> MSSVDVLLTVGKLDASLALLTTQDHHVIEFPTVLLPENVKAGSIIKMQVSQNLEEEKKQRNHFKSIQAKILEKYGTH;> MNLFWPSETKKQNEIPGGDYTPGNSPSVQKGYQFLNRDIFKSCPRIMERQFGECLHNRTHLIKDLISSGNVGLGPIEIVHMSYLNKHEKEEFGEYFYVTGIEVSGPAMPVEFLEVLKSSKRISKNISNNIILTYCCFNFFSNLDIRIRYDADDTFQTTAIDCNKETTDLTMTEKMWEETFASSVIRAIITNTNPELKPPGL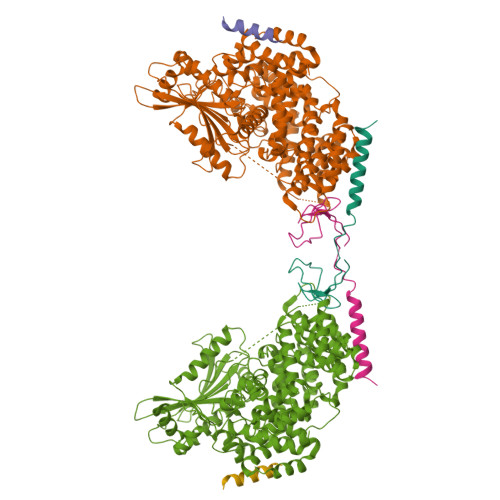VECPFYVGKDTISSCKKIIELLCRFLPRSLNCGWDSTKSMQATIVNNYLMYSLKSFIAITPSLVDFTIDYLKGLTKKDPIHDIYYKTAMITILDHIETKELDMITILNETLDPLLSLLNDLPPRDADSARLMNCMSDLLNIQTNFLLNRGDYELALGVSNTSTELALDSFESWYNLARCHIKKEEYEKALFAINSMPRLRKNDGHLETMYSRFLTSNYYKKPLNGTREHYDLTAMEFTNLSGTLRNWKEDELKRQIFGRIAMINEKKIGYTKEIWDDIAIKLGPICGPQSVNLINYVSPQEVKNIKNINLIARNTIGKQLGWFSGKIYGLLMEIVNKIGWNGLLNIRTEAFMMETEFYQASNNIIDENGHIPMESRKKRFCEGWLDDLFLDLYQDLKLSKISLSNKDEKHSGLEWELLGLIMLRTWHWEDAVACLRTSIVARFDPVSCQQLLKIYLQPPKNIQEVTLLDTDTIISLLIKKISYDCRYYNYCQIFNLQLLEKLCNELGTHILRNKILLQPSIGDEIMVMIDAMLAWIADLDHTVQPGTENLYFQGHHHHHH;> DDYYLNLNQDEESLLRSRC>[3x]MNLEVLCGRINVENGLSLGEPGLYDQIYDRPGLPDLDVTVDATGVTVDIGAVPDSASQLGSSINAGLITIQLSEAYKINHDFTFSGLSKTTDRRLSEVFPITHDGSDGMTPDVIHTRLDGTI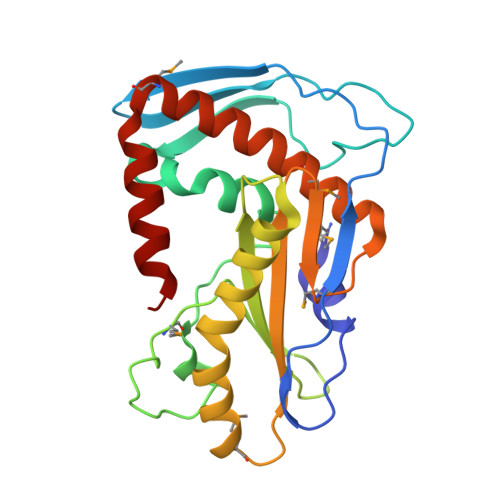VVVEFSTTRSHNIGGLEAAYRTKIEKYRDPISRRVDIMENPRVFFGVIVVSSGGVLSNMPLTQDEAEELMYRFCIANEIYTKARSMDADIELQKSEEELEAISR>GAMEVAVLAESELGSEAQRERRKRILDATMAIASKGGYEAVQMRAVADRADVAVGTLYRYFPSKVHLLVSALGREFSRIDAKTDRSAVAGATPFQRLNFMVGKLNRAMQRNPLLTEAMTR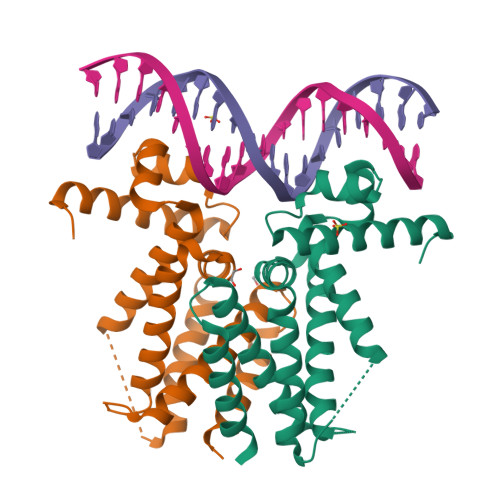AYVFADASAASEVDQVEKLIDSMFARAMANGEPTEDQYHIARVISDVWLSNLLAWLTRRASATDVSKRLDLAVRLLIGDQDSA[2x]> GPMENEQNNQDSENGLDYFRSMYDRYRDVFINHINDYVLEDDIKIIISKYYKLLFDYNCLGGKNNRGILVILIYEYVKNRDINCNEWEKVACIAWCIEILQASFLVADDIMDKGETRRNKHCWYLLKDVEIKNAVNDVFLLYNAIYKLLDVYLRNDNCYLDLITSFREATLKTIV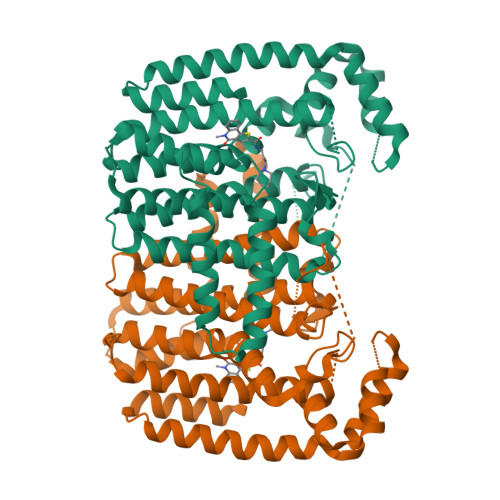GQHLDTNIFSDKYSHIDKDIDVNNINISQENKININMLNFKVYQNIIIHKTAYYSFFLPIVCGMQMGGISLDNLLYKKVENIAILMGEYFQVHDDYIDTFGDSKKTGKVGSDIQNNKLTWPLIKAFELCSQPEKEDIIRNYGKDNVTCIKFINDIYEHYNIRDHYVEYEKKQKMKILEAINQLHHEGIEYVLKYVMDILFTGA methyl (2S,3R)-1-(methanesulfonyl)-3-methylpiperidine-2-carboxylate 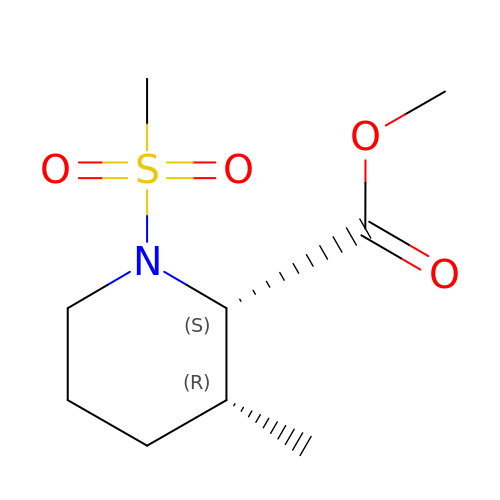| C9 H17 N O4 S | HLMYNIFJGFTOOM-SFYZADRCSA-N> SEILPFQYVLCAATSPAVKLHDETLTYLNQGQSYEIRMLDNRKLGELPELNGKLVKSIFRVVFHDRRLQYTEHQQLEGWRWNRPGDRILDIDIPMS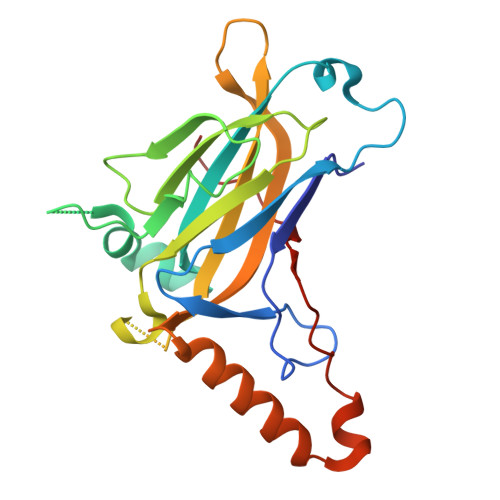VGVIDPRANPTQLNTVEFLWDPSKRTSVFIQVHCISTEFTMRKHGGEKGVPFRVQIDTFKENGNGEYTEHLHSASCQIKVFKPKGADRKQKIDREKMEKRTPHEKEKYQPSYETTILTECSPWPEI>ACYCRIPACIAGERRYGTCIYQGRLWAFCC[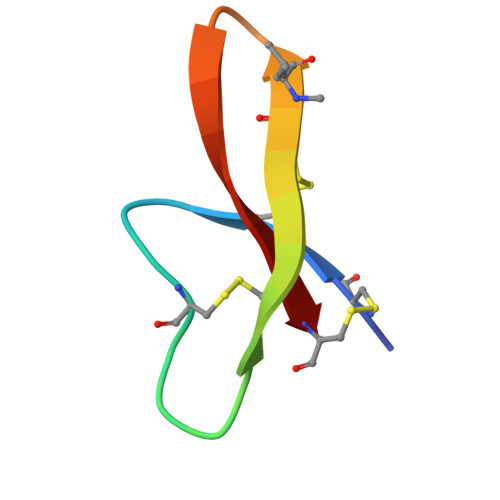2x]>GMPVNSILGVFAKSPIKPLQEHMDKVYDCASLLVPFFEATITGNWDDAVQIRKQISLAEKQGDSLKREIRLTLPSGLFMPVERTDLLELLTQQDKIANKAKDISGRVIGRQLLIPQALQVPFIAYLQ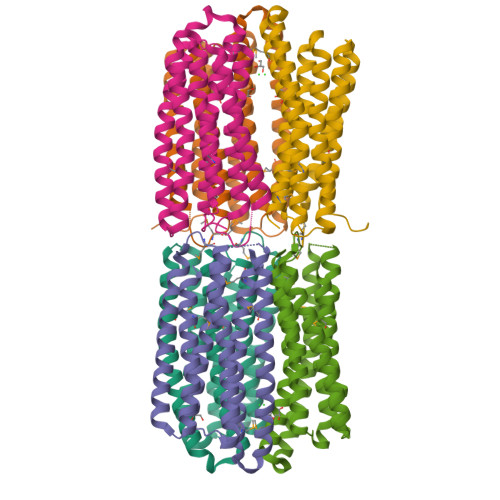RCIDAVGLAQQVINELDDLLEAGFRGREVDFVAKMINELDIIEEDTDDLQIQLRRQLFALESELNPVDVMFLYKTIEWVGGLADLAERVGSRLELMLARV[3x]> MTHGAVKTYGIRLRVWGDYACFTRPEMKVERVSYDVMPPSAARGILEA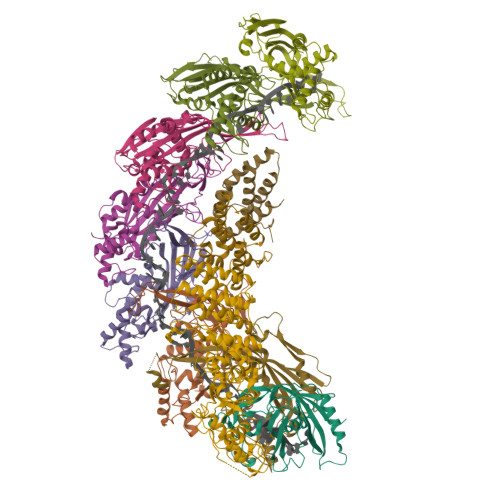IHWKPAIRWIVDRIHVLRPIVFDNVRRNEVSSKIPKPNPATAMRDRKPLYFLVDDGSNRQQRAATLLRNVDYVIEAHFELTDKAGAEDNAGKHLDIFRRRARAGQSFQQPCLGCREFPASFELLEGDVPLSCYAGEKRDLGYMLLDIDFERDMTPLFFKAVMEDGVITPPSRTSPEVRA;>[7x]MTAIANRYEFVLLFDVENGNPNGDPDAGNMPRIDPETGHGLVTDVCLKRKIRNHVALTKEGAERFNIYIQEKAILNETHERAYTACDLKPEPKKLPKKVEDAKRVTDWMCTNFYDIRTFGAVMTTEVNCGQVRGPVQMAFARSVEPVVPQEVSITRMAVTTKAEAEKQQGDNRTMGRKHIVPYGLYVAHGFISAPLAEKTGFSDEDLTLFWDALVNMFEHDRSAARGLMSSRKLIVFKHQNRLGNAPAHKLFDLVKVSRAEGSSGPARSFADYAVTVGQAPEGVEVKEML;> MILQALHGYYQRMSADPDAGMPPYGTSMENISFALVLDAKGTLRGIEDLREQEGKKLRPRKMLVPIAEKKGNGIKPNFLWENTSYILGVDAKGKQERTDKCHAAFIAHIKAYCDTADQDLAAVLQFLEHGEKDLSAFPVSEEVIGSNIVFRIEGEPGFVHERPAARQAWANCLNRREQGLCGQCLITGERQKPIAQLHPSIKGGRDGVRGAQAVASIVSFNNTAFESYGKEQSINAPVSQEAAFSYVTALNYLLNPSNRQKVTIADATVVFWAERSSPAEDIFAGMFDPPSTTAKPESSNGTPPEDSEEGSQPDTARDDPHAAARMHDLLVAIRSGKRATDIMPDMDESVRFHVLGLSPNAARLSVRFWEVDTVGHMLDKVGRHYRELEIIPQFNNEQEFPSLSTLLRQTAVLNKTENISPVLAGGLFRAMLTGGPYPQSLLPAVLGRIRAEHARPEDKSRYRLEVVTYYRAALIKAYLIRNRKLEVPVSLDPARTDRPYLLGRLFAVLEKAQEDAVPGANATIKDRYLASASANPGQVFHMLLKNASNHTAKLRKDPERKGSAIHYEIMMQEIIDNISDFPVTMSSDEQGLFMIGYYHQRKALFTKKNKEN;>[2x]VSLDPARTDRPYLLGRLFAVLEKAQEDAVPGANATIKDRYLASASANPGQVFHMLLKNASNHTAKLRKDPERKGSAIHYEIMMQEIIDNISDFPVTMSSDEQGLFMIGYYHQRKALFTKKNKEN> GSHMPESVIQNYNKALQQLEKYKPYEEALLQAEAPRLAEYQAYIDFEMKIGDPARIQLIFERALVENCLVPDLWIRYSQYLDRQLKVKDLVLSVHNRAIRNCPWTVALWSRYLLAMERHGVDHQVISVTFEKALNAGFIQATDYVEIWQAYLDYLRRRVDFKQDSSKELEELRAAFTRALEYLKQ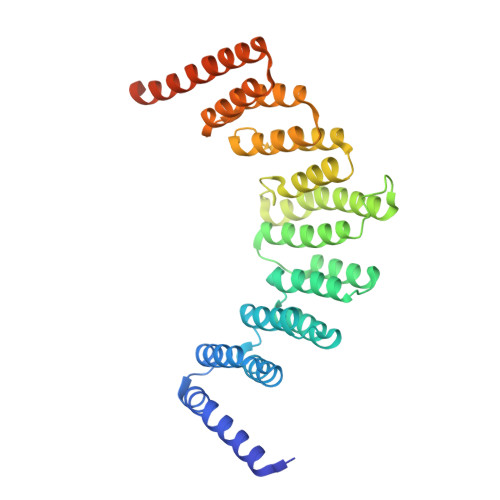EVEERFNESGDPSCVIMQNWARIEARLCNNMQKARELWDSIMTRGNAKYANMWLEYYNLERAHGDTQHCRKALHRAVQCTSDYPEHVCEVLLTMERTEGSLEDWDIAVQKTETRLARVNEQRMKAAEKEAALVQQEEEKAEQRKRARAEKKAL The protein at the heart of both T3SS secretion and secretion specificity belongs to the SctV/FlhA family (injectisome and flagellar system names respectively). While only injectisome members have been given unified Sct names, the SctV/FlhA family is conserved across all T3SSs of both flagella and injectisomes, which assembles early into the inner membrane, and is central to T3SS assembly and function. The ~75 kDa SctV is composed of an N-terminal transmembrane domain functioning as a proton-protein antiporter export gate, and a C-terminal cytoplasmic domain (SctVC) implicated in funneling selected substrates to the export gate. SctVC’s substrate specificity is mediated by a trimeric “gatekeeper” complex (Portaliou et al., 2017, Yu et al., 2018) formed of SctW (in SPI-2, SsaL) and a heterodimeric chaperone (in SPI-2, SsaM and SpiC, lacking unified Sct nomenclature).

In the SPI-2 T3SS, SctV is often referred to by its original species-specific name SsaV; here we call it SctVSPI-2. To better understand the role of SctV in SPI-2 translocon-effector specificity switching, we purified full-length SctV and determined its toroidal cytoplasmic region’s structure using cryo-EM. Central to specificity switching is a nonameric SctV protein with an N-terminal transmembrane domain and a toroidal C-terminal cytoplasmic domain. Structural comparisons and molecular dynamics simulations revealed that the cytoplasmic torus is stabilized by its core subdomain 3, about which subdomains 2 and 4 hinge, varying the flexible outside cleft implicated in gatekeeper and substrate binding. SctVSPI-2 also features a short C-terminal extension not found in other branches of the SctV protein family, apparently required for efficient control of substrate specificity by the gatekeeper. In light of patterns of surface conservation, deprotonation, and structural motion, the location of previously identified critical residues suggest that gatekeeper binds a cleft buried between neighboring subdomain 4s. Simulations suggest that a local pH change from 5 to 7.2 stabilizes the subdomain 3 hinge and narrows the central aperture of the nonameric torus. Our results are consistent with a model of local pH sensing at SctV, where pH-dependent dynamics of SctV cytoplasmic domain affect binding of gatekeeper complex.

> MRSWLGEGVRAQQWLSVCAGRQDMVLATVLLIAIVMMLLPLPTWMVDILITINLMFSVILLLIAIYLSDPLDLSVFPSLLLITTLYRLSLTISTSRLVLLQHNAGNIVDAFGKFVVGGNLTVGLVVFTIITIVQFIVITKGIERVAEVSARFSLDGMPGKQMSIDGDLRAGVIDADHARTLRQHVQQESRFLGAMDGAMKFVKGDTIAGIIVVLVNIIGGIIIAIVQYDMSMSEAVHTYSVLSIGDGLCGQIPSLLISLSAGIIVTRVPGEKRQNLATELSSQIARQPQSLILTAVVLMLLALIPGFPFITLAFFSALLALPIILIRRKKSVVSANGVEAPEKDSMVPGACPLILRLSPTLHSADLIRDIDAMRWFLFEDTGVPLPEVNIEVLPEPTEKLTVLLYQEPVFSLSIPAQADYLLIGADASVVGDSQTLPNGMGQICWLTKDMAHKAQGFGLDVFAGSQRISALLKCVLLRHMGEFIGVQETRYLMNAMEKNYSELVKELQRQLPINKIAETLQRLVSERVSIRDLRLIFGTLIDWAPREKDVLMLTEYVRIALRRHILRRLNPEGKPLPILRIGEGIENLVRESIRQTAMGTYTALSSRHKTQILQLIEQALKQSAKLFIVTSVDTRRFLRKITEATLFDVPILSWQELGEESLIQVVESIDLSEEELADNEEHHHHHH>[2x]MQVKPCTPEFYQTHFQLAYRLQSRPRGLALVLSNVHFTGEKELEFRSGGDVDHSTLVTLFKLLGYDVHVLCDQTAQE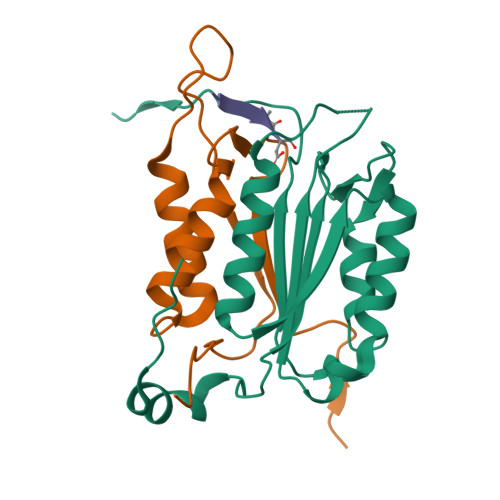MQEKLQNFAQLPAHRVTDSCIVALLSHGVEGAIYGVDGKLLQLQEVFQLFDNANCPSLQNKPKMFFIQACRGDETDRGVDQQD;>[2x]GKEKLPKMRLPTRSDMICGYACLKGTAAMRNAKRGSWYIEALAQVFSERACDMHVADMLVKVNALIKDREGYAPGTEFHRCKEMSEYCSTLCRHLYLFPGHPPTLEHHHHHH;>[2x]XVDVAD> GSAPSVKGVSFDQANNLLIEPARIEEEELTLTILRQTGGLGISIAGGKGSTPYKGDDEGIFISRVSEEGPAARAGVRVGDKLLEVNGVALQGAEHHEAVEALRGAGTAVQ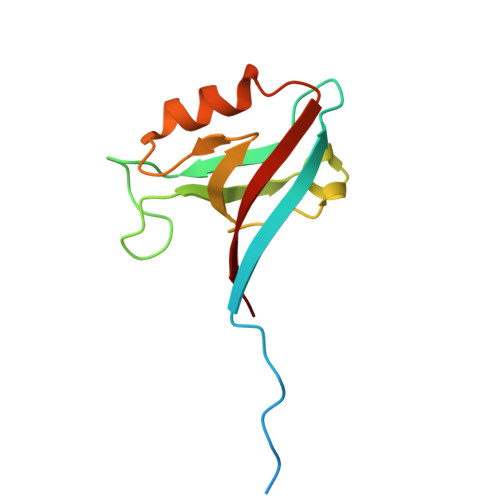MRVWRERM>[2x]MAPSRKFFVGGNWKMNGRK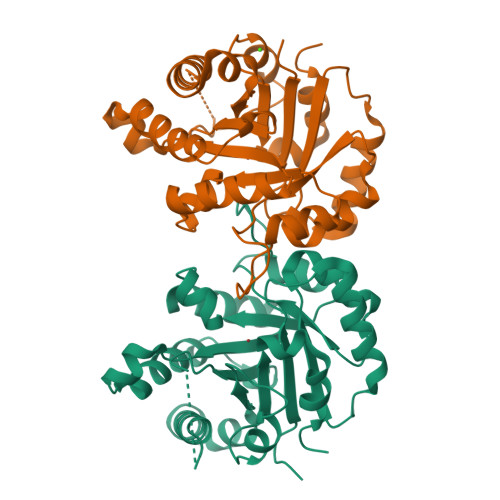QSLGELIGTLNAAKVPADTEVVCAPPTAYIDFARQKLDPKIAVAAQNCYKVTNGAFTGEISPGMIKDCGATWVVLGHSERRHVFGESDELIGQKVAHALAEGLGVIACIGEKLDEREAGITEKVVFEQTKVIADNVKDWSKVVLAYEPVWAIGTGKTATPQPAQEVHEKLRGWLKSNVSDAVAQSTRIIYGGSVTGATCKELASQPDVDGFLVGGASLKPEFVDIINAKQ>[2x]SRHSEKIAIRDFQVGDLVLIILDERHDNYVLFTVSPTLYFLHSESLPALDLKPGEGASGASRRPWVLGKVMEKEYCQAKKAQNRFKVPLGTKFYRVKAVSWNKKV;>[2x]SSGTSSEFEVV

Recent findings revealed that TNIP1 functions as a checkpoint mechanism that fine-tunes the rate of mitophagy by disrupting the recycling of the ULK complex during autophagosome formation. The phosphorylation of the TNIP1 FIR motif enhances its binding affinity for FIP200, enabling TNIP1 to compete with other autophagy receptors, such as CCPG1 or Optineurin. Here, we determined several crystal structures of the FIP200 claw domain in complex with phosphorylated TNIP1 FIR peptides and elucidated the specific recognition of different phosphorylated TNIP1 by FIP200 claw domain. Each FIP200 claw domain within the dimer features a five-stranded antiparallel β-sheet and a short α-helix.

TBK1 phosphorylates both S122 and S123 in the TNIP1 FIR motif, which is crucial for affecting the binding affinity for FIP200 (18). Phosphorylation on either S122 or S123 enhanced the binding affinity between the FIP200 claw domain and TNIP1 peptides. The binding affinity of FIP200 claw domain to the TNIP1_pS122pS123 peptide did not increase as expected, when compared with the TNIP1_pS123 peptide. For FIP200–TNIP1_pS122pS123 complex, due to the electrostatic repulsion between the phosphorylated S122 and S123 residues, the side chain of K1569 did not form additional direct hydrogen bonds with the phosphate group of TNIP1 pS123. Consequently, the expected enhancement of the binding affinity between the FIP200 claw domain and the TNIP1_pS122pS123 peptide did not occur as anticipated. In addition, unlike pattern II, the cumulative phosphorylation of the TNIP1 FIR motif does not enhance its binding affinity to FIP200 claw domain. This may because excessive phosphorylation in TNIP FIR leads to electrostatic repulsion and structural instability, as shown in FIP200–TNIP1_pS122pS123 complex.>[2x]MGHHHHHHHHHHSSGHIEGRHMRVIRVGTRKSQLARIQTDSVVATLKASYPGLQFEIIAMSTTGDKILDTALSKIGEKSLFTKELEHALEKNEVDLVVHSLKDLPTVLPPGFTIGAICKRENPHDAVVFHPKFVGKT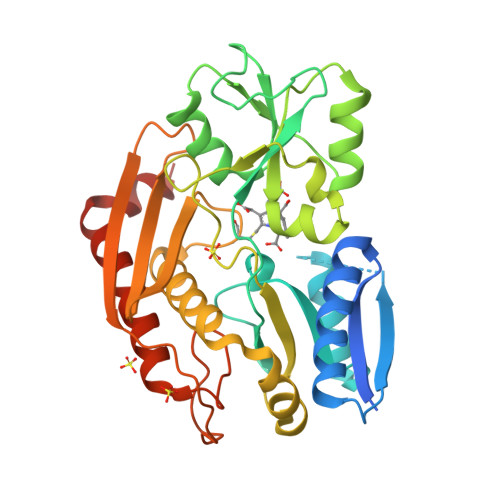LETLPEKSVVGTSSLRRAAQLQRKFPHLEFRSIRGNLNTRLRKLDEQQEFSAIILATAGLQRMGWHNRVGQILHPEECMYAVGQGALGVEVRAKDQDILDLVGVLHDPETLLRCIAERAFLRHLEGGCSVPVAVHTAMKDGQLYLTGGVWSLDGSDSIQETMQATIHVPAQHEDGPEDDPQLVGITARNIPRGPQLAAQNLGISLANLLLSKGAKNILDVARQLNDAH> MEIPPEISHALSEIGFTKYEILTYWTLLVYGPSTAKEISTKSGIPYNRVYDTISSLKLRGFVTEIEGTPKVYAAYSPRIAFFRFKKELEDIMKKLEIELNNVKKEEQRPAIWRSRSFDEAIEMFRESLYSAKNEVIVVTPSEFFETIREDLIKTLERGVTVSLYIDKIPDLSEFKGKGNFFVRQFYKLNHLIGMTDGKEVVTIQNATFDSIGPPSFKSTYPEIIFSQYSLIIEIFKESTLEKEIIGNPKDIRFFAMFHAVDFVKNHLKNRNIYAEITGKNLESGRLETLTGRVVGYTL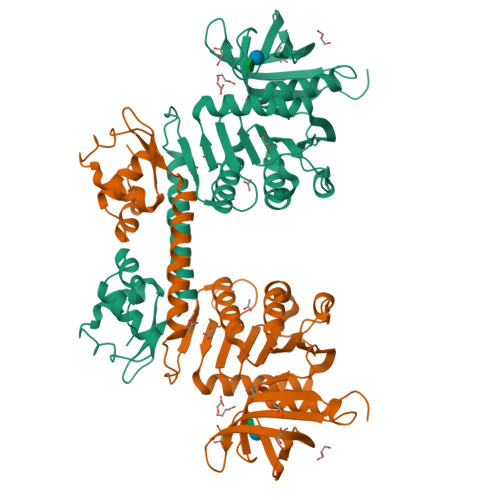SLREAVNNIHLETENGVVKVGGMFAVIEDYESTEIKFIMGVDLQ> GPPGPKGPKGDPGDPGPPGARGQAGVLGFPGPPGPKGPKGDPGDPG;> XGPPGPPG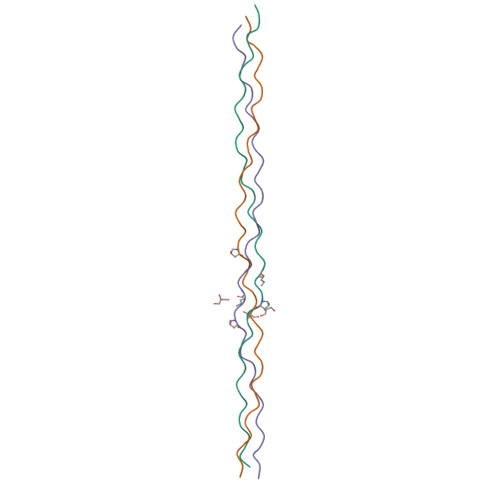DKGDKGPPGPPGARGEPGNIGFPGPPGPPGDKGDKGPPG;> XGPPGPKGPKGDPGDPGPPGARGQAGVLGFPGPPGPKGPKGDPGDP> SVSKTSQTDKDEDNLDFTKNLLTRIKNLHPLTNKSTIHSLLSYVFSRQTQNIACEPMYIDYRKDETEAIIRWKTPLHAETCINAFRTQERKQNSHDDIRAHRKKGSSRPFLIAELITGE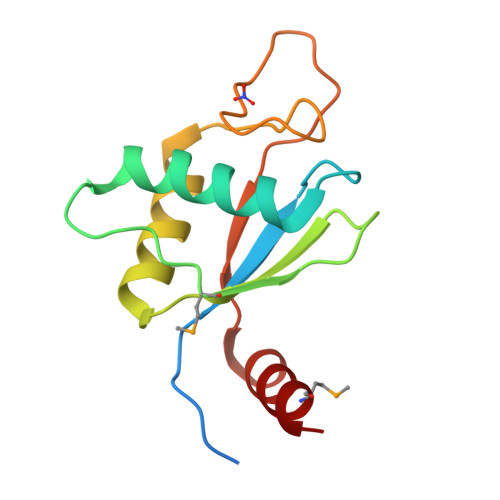EEKNYWRMLKK>GTNAAMRKAFNYQDTAKNGKKCSGCAQFVPGASPTAAGGCKVIPGDN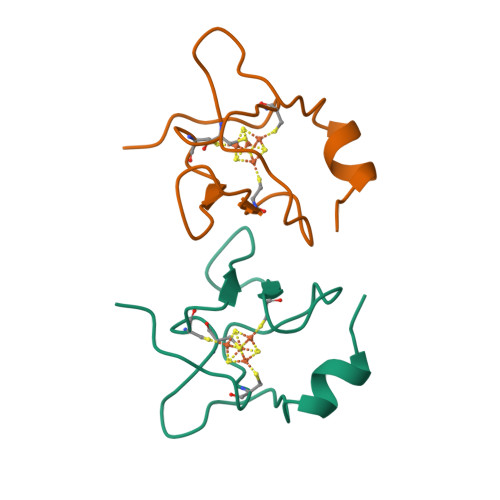QIAPGGYCDAFIVKK[2x]>MPGYTNMEKQAIARQYLWPKQVRESGMEGRIEVTDAAILRVISEYTREAGVRGLERELGKIARKGAKFWLEGAWEGLRTIDASDIPTYLGIPRYRPDKAETEPQVGTAQGLAWTPVGGTLLTIEVAAVPGSGKLSLTGQLGEVMKESAQAALTYLRAHTQDYGLPEDFYNKVDLHVHVPDGATPK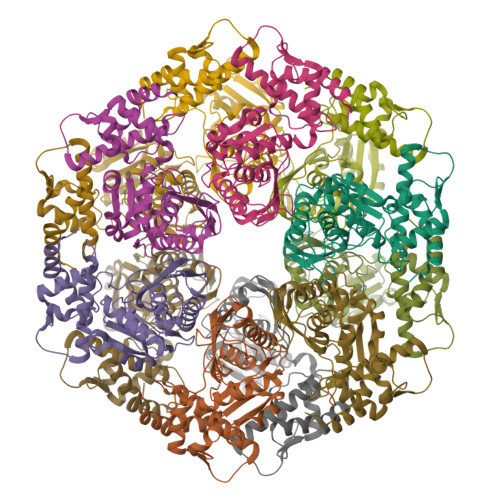DGPSAGITMATAIASALSRRPARMDIAMTGEVSLRGKVMPIGGVKEKLLAAHQAGIHKIVLPKDNEAQLEELPKEVLEGLEIKLVEDVGEVLEYLLLPEPTMPPVVQHHHHHH[12x]> MILVGIAVLILLAVFAILYYKQKEKFVVVGKFVEPIPSNPGQDFTLLPMDQTYTFADPVP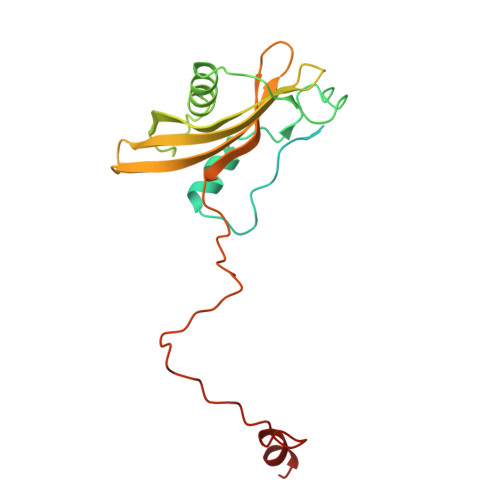DTATAFDVVLSRFTDKKAPADLLKGATFPEAAPYTDSEVENISKLALSRVKGPDAPVLSFISVEYAAKGVDNKKNTHYDIAFMVYDQVKNFSLKLVLVAVLDAKNKLWIKKFSSFNSFTPKDKGPKGVENIDETPLAEFIPDFVQFSRLYKDNANV> APIERPEDFLKDKEKAKEWERKEAERIEQKLERSEKEALESYKKDSVEISKYSQTRNYFYDYQIEANSREKEYKELRNAISKNKIDKPMYVYYFESPEKFAFNKVIRTENQNEISLEKFNEFKETIQNKLFKQDGFKDISLYEPGKGDEKPTPLLMHLKLPRNTGMLPYTNTNNVSTLIEQGYSIKIDKIVRIVIDGKHYIKAEASVVSSLDFKDDVSKGDSWGKANYNDWSNKLTPNELADVNDYMRGGYTAINNYLISNGPVNNPNPELDSK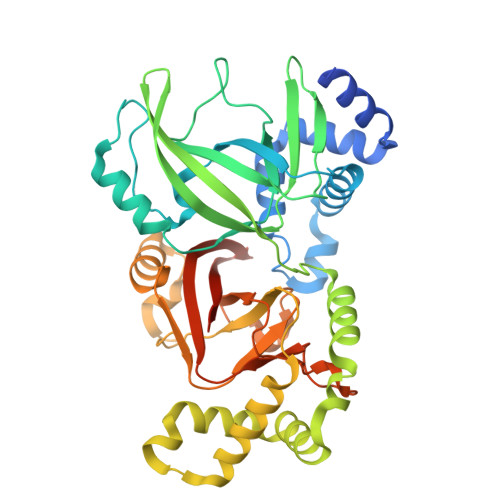ITNIENALKREPIPTNLTVYRRSGPQEFGLTLTSPEYDFNKLENIDAFKSKWEGQALSYPNFISTSIGSVNMSAFAKRKIVLRITIPKGSPGAYLSAIPGYAGEYEVLLNHGSKFKINKIDSYKDGTITKLIVDATLIPENLYFQGLEHHHHHH> MASMTGGQQMGRGSMAGVLPAHGTQHGIRLPLRSGLGGAPLGLRLPRETDEEPEEPGKKGSFVEMVDNLRGKSGQGYYVEMTVGSPPQTLNILVDTGSSNFAVGAAPHPFLHRYYQRQLSSTYRDLRKGVYVPYTQGKWEGELGTDLVSIPHGPNVTVRANIAAITESDKFFINGSNWEGILGLAYAEIARPDDSLEPFFDSLVKQTHVPNLFSLQLCGAGFPLNQSEVLASVGGSMIIGGIDHSLYTGSLWYTPIRREWYYEVIIVRVEINGQDLKMDCKEYNYDKSIVDSGTTNLRLPKKVFEAAVKSIKAASSTEKFPDGFWLGEQLVCWQAGTTPWNIFPVISLYLMGEVTNQSFRITILPQQYLRPVEDVATSQDDCYKFAISQSSTGTVMGAVIMEGFYVVFDRARKRIGFAVSACHVHDEFRTAAVEGPFVTLD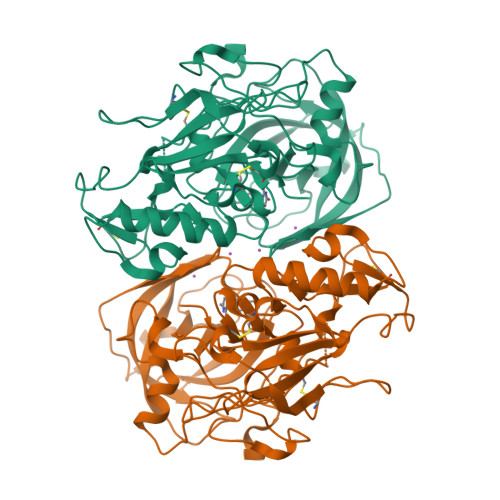MEDCGYNIPQTDES>GDADVLVKWSEDLANLPSIDTQHKRLVDYINDLYRAARRRDMDKAREVFDALKNYAVEHFGYEERLFADYAYPEATRHKEIHRRFVETVLKWEKQLAAGDPEVVMTTLRGLVDWLVNHHMKEDKKYEAYLRERGVS[2x]

Despite these functional differences, all of these proteins have a carboxylate-bridged diiron active site within a four-helix bundle protein folding motif.2a,6 The coordination sphere and the environment surrounding the diiron site in these proteins have apparently evolved to optimize a variety of reactions with O2. As a target protein for engineering the coordination sphere, we have selected DcrH-Hr,8 which contains the histidine-rich coordination sphere and exhibits spectroscopic properties characteristic of all Hrs, but contains a larger substrate-accessible tunnel within the four-helix bundle compared to classical Hrs. As for classical Hrs, the diiron site of DcrH-Hr reversibly binds O2 but shows more rapid autoxidation. Herein, we report another engineered variant DcrH-Hr, I119H, of the same residue, in which alteration of the coordination sphere generates the capability of H2O2-dependent oxidation of exogenous substrates.

I119H was expressed from Escherichia coli and purified as a holo-form containing approximately 1.6 iron atoms per protein, as determined by ferrozine analysis. The diferric form (met-I119H) exhibited two absorption maxima at 325 and 375 nm, which are well-established to arise from oxo to ferric LMCT transitions in the oxo–dicarboxylate-bridged met-Hrs.1b,c,8 Resonance Raman (rR) spectra of I119H gave a characteristic peak at 499 cm–1 for the symmetric stretching Fe–Ooxo–Fe vibrational mode. The met-I119H protein was crystallized, and the structure of the oxo-bridged diiron site13 was determined by X-ray crystallographic analysis at a resolution of 1.9 Å. The overall structure of the met-I119H is similar to that of the met form of WT (met-WT) (RSMD value, 0.324).10 Surprisingly, H119 coordinates to Fe1 in the crystal structure in place of the conserved H118 ligand residue in WT. The coordination geometry of other His residues and carboxylate ligands is almost identical to that of met-WT (ESI†). A computational study of the I119H diiron site yielded alternative structures in which either H118 or H119 coordinates to the Fe1.14 It is, thus, expected that either H118 or H119 coordination would be stable in I119H in solution. Based on this observation together with the crystal structure and calculated optimized structures, we propose two conformations for I119H: H118off/H119on and H118on/H119off. In the latter case, the H119 residue is capable of forming a hydrogen bonding interaction with an exogenous ligand. Motivated by the differing reactivity of WT and I119H toward H2O2, we tested the promotion of oxidation of external substrates by these proteins. Fig. 4b demonstrates that I119H promotes oxidation of guaiacol by H2O2, as shown by the clear increase in absorption at 470 nm assigned to the oxidized guaiacol product, whereas, under the same conditions, WT does not.2-(3,4,5-TRIHYDROXY-PHENYL)-CHROMAN-3,5,7-TRIOL | C15 H14 O7 | 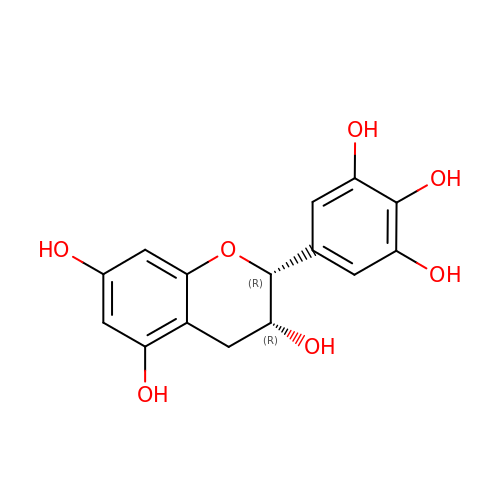XMOCLSLCDHWDHP-IUODEOHRSA-N> MDGAGAEEVLAPLRLAVRQQGDLVRKLKEDKAPQVDVDKAVAELKARKRVLEAKELALQPKDDIVDRAKMEDTLKRRFFYDQAFAIYGGVSGLYDFGPVGCALKNNIIQTWRQHFIQEEQILEIDCTMLTPEPVLKTSGHVDKFADFMVKDVKNGECFRADHLLKAHLQKLMSDKKCSVEKKSEMESVLAQLDNYGQQELADLFVNYNVKSPITGNDLSPPVSFNLMFKTFIGPGGNMPGYLRPETAQGIFLNFKRLLEFNQGKLPFAAAQIGNSFRNEISPRSGLIRVREFTMAEIEHFVDPSEKDHPKFQNVADLHLYLYSAKAQVSGQSARKMRLGDAVEQGVINNTVLGYFIGRIYLYLTKVGISPDKLRFRQHMENEMAHYACDCWDAESKTSYGWIEIV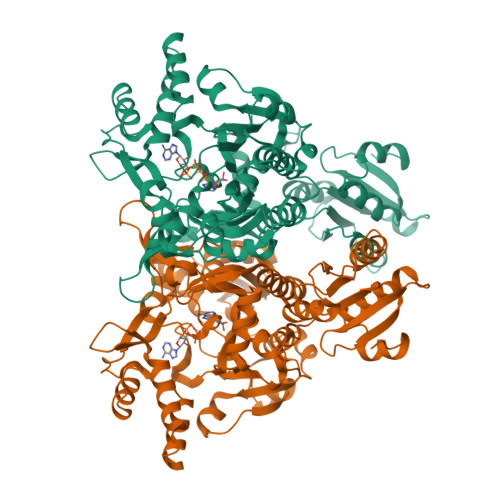GCADRSCYDLSCHARATKVPLVAEKPLKEPKTVNVVQFEPSKGAIGKAYKKDAKLVMEYLAICDECYITEMEMLLNEKGEFTIETEGKTFQLTKDMINVKRFQKTLYVEEVVPNVIEPSFGLGRIMYTVFEHTFHVREGDEQRTFFSFPAVVAPFKCSVLPLSQNQEFMPFVKELSEALTRHGVSHKVDDSSGSIGRRYARTDEIGVAFGVTIDFDTVNKTPHTATLRDRDSMRQIRAEISELPSIVQDLANGNITWADVEARYPLFEGQETGKKETIEELEHHHHHH>MRRYEVNIVLNPNLDQSQLALEKEIIQRAAENYGARVEKVEELGLRRLAYPIAKDPQGYFLWYQVEMPEDRVNDAARELRIRDNVRRVMVVKSQEP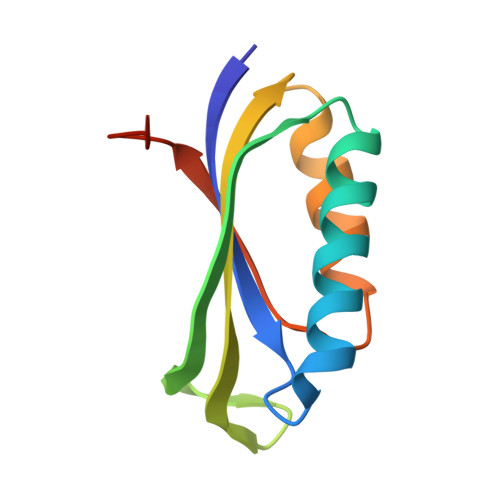FLANA[2x]> SEKNGAHSFLS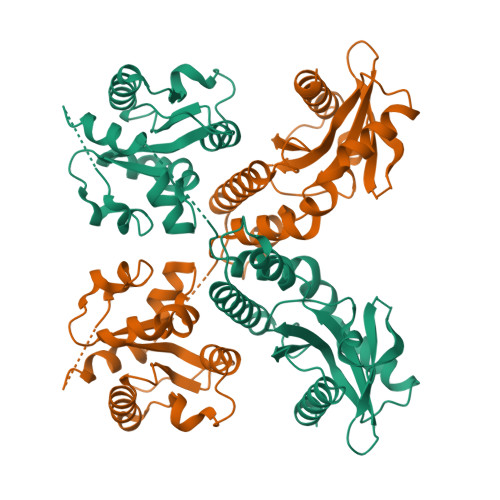DTPVTSLTMSVPVLRHPHVYHAFISYCADADTSHARTILDSVESRGFTCCFAERDFLPGECTSDVVVDAIHCSKNVILVISPASLQSEWSKFEMLMAVDDSHQRNNVCLVPVLLGGVKVDDLPPPLRPLTCIELMDDFRNTDDIIQAISKPEDTWESLLPVGNLAHGFAWGYYYGYLKIILPDLDKTVRQWRRVNNAEGRMSEKLFLFFPQSCRCRDSIADESSLIKHRGHLPIITKDRAGIIERQYKNTIYSVTDDNGEDYFFAGEYIGVIHTMFEMEQNATTGLQTREKYVQSMRFYLTLKRILDTDPECSKKCKIVFYKDVNNSSDAMPRLICNEIKNQLRKESSDDTTVCMTPFNSPFPSISSPDFARCSLKSSSSTNMVKSEPNIYREESGKTKSVERG> MASVPQLLDDLCEALLPAAKAHLGQRRGSRKRAKQSLKKVAYNALFTNLFQDEARKLQPDLPRLPVKNRILMLSFDLRVGGLAAEADRLEELVEGLETAPRGPLAELGSVLDLLVQLAGSGPPRVLQRRRDYFLPKEHVGRNVRYGGYDCCHLSGIEADVRSIISGEEELCRDLIRKTLQVMEAAPGTGLPAFGLSSYGDPYGDRFERDTRVSLFGALVHSRTADLDVRLDLPPVPDSADVSGLAIKVPLSVDQSEDEGFQSAPNLTPDSQSEPGVTPDIDLWEAVLTYEASRRRCWEQIGCPPGHREEPYLTEAGRDAFDRFCRLRQGELQVLGGALLQAPQPVLVKESELVKDTLNVLLGVVSATFSLCQPAQAFTVKRGVHVSGASPESVSSLLSEVAECGTHYARLSDFSLQPVLDSSCSKGLVFQAFTSGLRRYLQYYRACVLSTPPTLSLLTIGFLFKKLGRQLRYLAELCGVGTALPGTGGGEPRAAFPTGVRLLSYLYQEALDNCSNEHYPVLLSLLKTSCEPYTRFIHDWVYSGVFRDVYGEFMIQVNHEYLGCRDKSYWTHGYVLVSKEVEACVPVFLKHVAHDVYVCGKTINLLKLCCPRHYLCCSDVPVPRISVIFSLEELKDIEKDCAIYVGRMERVARHSSLSKEEKELRMEIAKQELIVHAREAASRVLSALSDRQMSERMALDARKREQFQRLKEQFMRDQERRRAARQEELDDDFSYARELRDRERRLKALEEQLERKARQALVDHYSKLSAEAARRERKALWRVQRHRLADARRRFLLEEEKRVQVMPSCSWERNQGALVFQASLPCPEHPDGGGGCGSGPSEQPKAARDGPRGPSRLMPQLPESPAEAACGLLSVGLSIRDFLPTAQGAEQPLHTGSALVLEEALQTIGSDLPPPAPSAAVGTGPSGPQEYDFRTILRPAVATSAFPGPLQSTGGGLGSEGQPQWEDTHVQLDMCVLDGQVALPHACSPQKTSPQEGSQAMGQLLRQVSEGD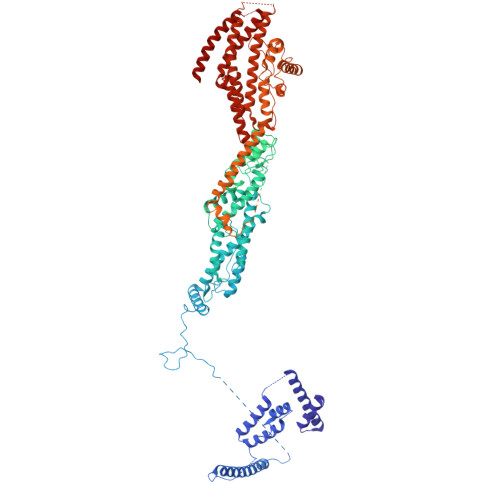VPTGGYASGTAPSRPRWNVHGHVSDASIKVGENVCDVVPSRPRWNVHGHVSDASIKVGENVCDVVPSRPRWNVHGHVSDASIKVGENVCDVVPSRPRWNIHGHVSDASIKVGENVCDVVPSRPRWNVHGHVSQSQVTLGVLSGEAEPIVPWPHQTPPDHGSQSGLSLGAQSPAQEGEPQPAAETAVEGAESGPQASPTAGAGSSLLSGSRLGPEARPPPPPPHLFCPGRSEDTVDLPASCRPSSQVRGQGLGVGGESSAGCPSHPACPFMGNEGSVPGPGVDTQSSPGLGEEAAQRWGMEQAYLAGLAGQYRLEQYPDSYEAMSEPPVARLLHHGLPRAFALPEDSGVQPDTDETAVQLSELLPLPVLMKHSVTAPLAAHVSLVNKAAVDYFFVELHLGAHFEALRHFLLMEDGEFAQSLSDLLFEKLGAGQTPGELLSPLVLNSVLSKALQYSLHGDTPHAANLSFALKFLPEAFAPNAPDVLSCLELRYKVDWPLNIVVTEGCLSRYSGIFSFLLQLKLMMWTLKDVCFHLKRTARMSHVASSVQFRQLQLFKHEMQHFVKVIQGYIANQILHVTWCEFRARLASVGDLEEIQRAHAEYLHKAVFRGLLTEKAAPAMNIIHSLFSLVLKFRSQLISQPWGLAGGPHGAEHPNFALMQQSYSTFKYYSHFLFKVVSKLVNRGYQPHLEDFLLRINFNNYYQDA> QAKHKQRKRLKSSCKRHPLYVDFSDVGWNDWIVAPPGYH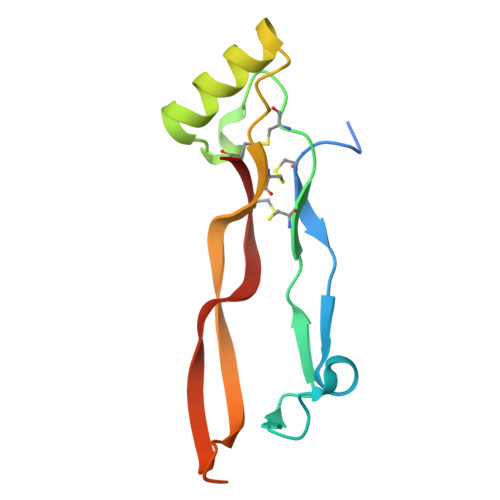AFYCHGECPFPLADHLNSTNHAIVQTLVNSVNSKIPKACCVPTELSAISMLYLDENEKVVKKDYQDMVVEGCGCR> MTKNQALRAALDSGRLFTAMAAHNPLVAKLAEQ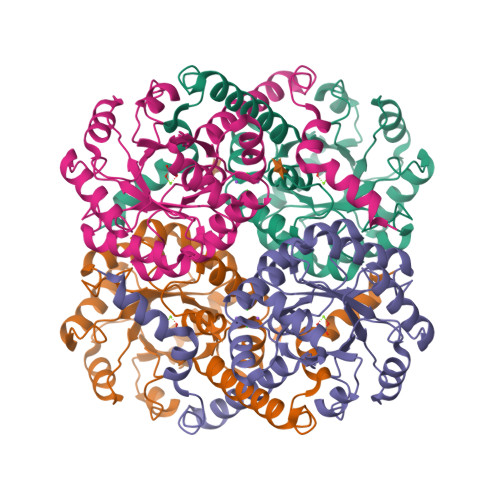AGFGGIWGSGFELSASYAVPDANILSMSTHLEMMRAIASTVSIPLIADIDTGFGNAVNVHYVVPQYEAAGASAIVMEDKTFPKDTSLRTDGRQELVRIEEFQGKIAAATAARADRDFVVIARVEALIAGLGQQEAVRRGQAYEEAGADAILIHSRQKTPDEILAFVKSWPGKVPLVLVPTAYPQLTEADIAALSKVGIVIYGNHAIRAAVGAVREVFARIRRDGGIREVDAALPSVKEIIELQGDERMRAVEARYLK>[2x]MDSVCPQGKYIHPQNNSICCTKCHKGTYLYND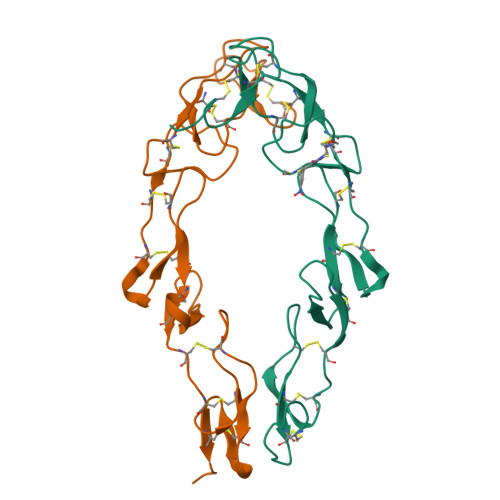CPGPGQDTDCRECESGSFTASENHLRHCLSCSKCRKEMGQVEISSCTVDRDTVCGCRKNQYRHYWSENLFQCFNCSLCLNGTVHLSCQEKQNTVCTCHAGFFLRENECVSCSNCKKSLECTKLCLPQIEN> XMYQQDQVVKEDNIEAVGKKLHEYNTQFQEKSREYDRLYEDYTRTSQEIQMKRTAIEAFNETIKIFEEQCQTQERYSKEYIEKFKREGNETEIQRIMHNYEKLKSRISEIV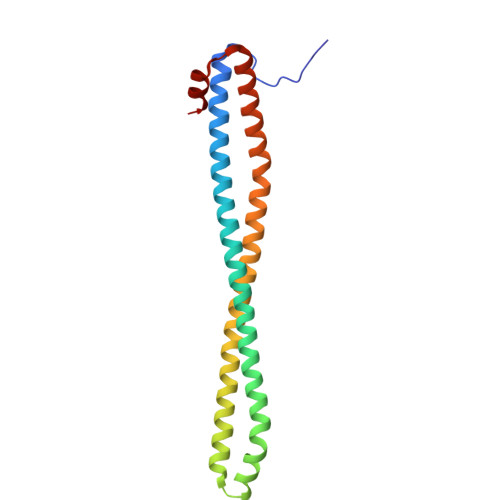DSRRRLEEDLKKQAAEYREIDKRMNSIKPDLIQLRKTRDQYLMWLTQKGVRQKKLNEWLGN> MASKPQPIAAANWKCNGSESLLVPLIETLNAATFDHDVQCVVAPTFLHIPMTKARLTNPKFQIAAQNAGNADALASLKDYGISWVVLGHSERRLYYGETNEIVAEKVAQACAAGFHVIVCVGETNEEREAGRTAAVVLTQLAAVAQKLSKEAWSRVVIAYEPVWAIGTGKVATPQQAQEVHELLRRWVRSKLGTDIAAQLRILYGGSVTAKNARTL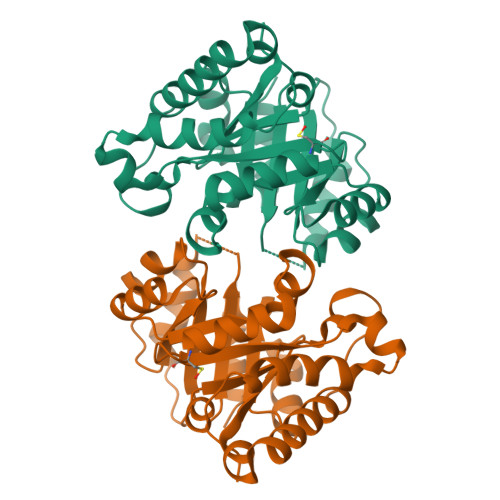YQMRDINGFLVGGASLKPEFVEIIEATK> GIDPFTMTRKARTPKAAPVPEAVAVVEPPPPDAAPTGPRLSRLEIRNLATITQLELELGGGFCAFTGETGAGKSIIVDALGLLLGGRANHDLIRSGEKELLVTGFWGDGDESEADSASRRLSSAGRGAARLSGEVVSVRELQEWAQGRLTIHWQHSAVSLLSPANQRGLLDRRVTKEAQAYAAAHAAWREAVSRLERLQASQRERARQIDLLAFQVQEISEVSPDPGEEEGLNTELSRLSNLHESSKHPTSLVPRGSGSAADPEALDRVEARLSALSKLKNKYGPTLEDVVEFGAQAAEELAGLEEDERDAGSLQADVDALHAELLKVGQALDAAREREAEPLVDSLLAVIRELGMPHA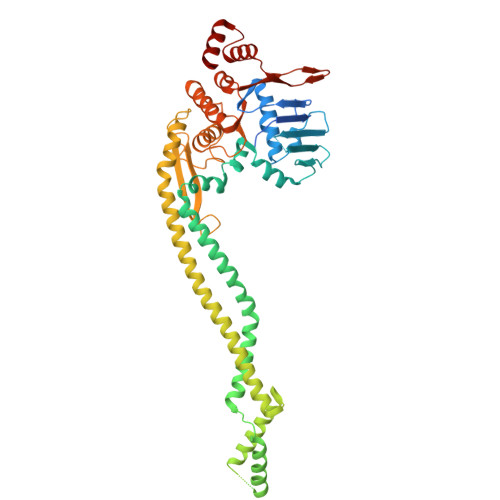RMEFALSALAEPAAYGLSDVLLRFSANPGEELGPLSDVASGGELSRVMLAVSTVLGADTPSVVFDEVDAGIGGAAAIAVAEQLSRLADTRQVLVVTHLAQIAARAHHHYKVEKQVEDGRTVSHVRLLTGDERLEEIARMLSGNTSEAALEHARELLAG> KNADSYAKKPHISALNAPQLDQRYKNEFTIGAAVEPYQLQNEKDVQMLKRHFNSIVAENVMKPISIQPEEGKFNFEQADRIVKFAKANGMDIRFHTLVWHSQVPQWFFLDKEGKPMVNETDPVKREQNKQLLLKRLETHIKTIVERYKDDIKYWDVVNEVVGDDGKLRNSPWYQIAGIDYIKVAFQAARKYGGDNIKLYMNDYNTEVEPKRTALYNLVKQLKEEGVPIDGIGHQSHIQIGWPSEAEIEKTINMFAALGLDNQITELDVSMYGWPPRAYPTYDAIPKQKFLDQAARYDRLFKLYEKLSDKISNVTFWGIADNHTWLDSRADVYY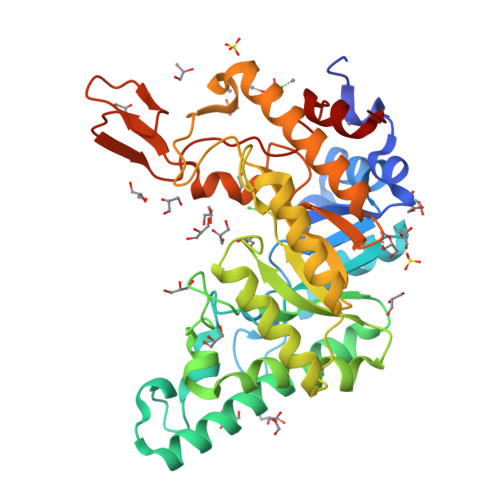DANGNVVVDPNAPYAKVEKGKGKDAPFVFGPDYKVKPAYWAIIDHK> GHMLEPETTLNDKQDSTDLKVKVSAKISSIINYNEGQWSPNNPSGKKQYDREQLLQLREVKASRIQPEVKNVSILP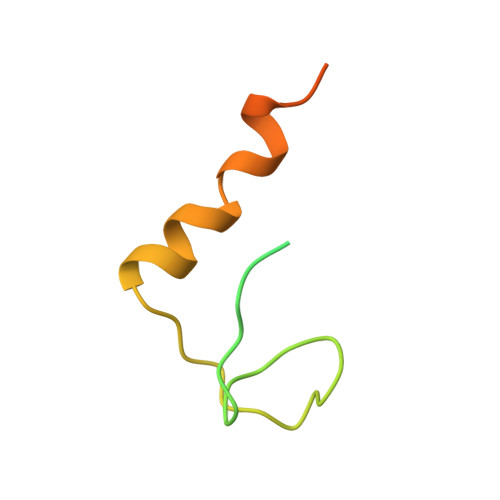QP Caprolactamase is the first enzyme in the caprolactam degradation pathway of Pseudomonas jessenii. It is composed of two subunits (CapA and CapB) and sequence‐related to other ATP‐dependent enzymes involved in lactam hydrolysis, like 5‐oxoprolinases and hydantoinases. Activity assays with lysates of Escherichia coli cells producing these proteins indicated they are subunits of a caprolactamase (EC 3.5.2.‐x) that catalyzes the first step in the catabolic pathway: the ATP‐dependent hydrolysis of the lactam ring to form 6‐aminocaproic acid (6‐ACA). The crystal structure of caprolactamase shows an (α/β)2 tetramer, with the α subunits (CapA) responsible for ATP‐dependent substrate phosphorylation and the β subunits (CapB) for hydrolytic lactam ring opening.

A 4.0 Å resolution dataset was collected from a single crystal grown in phosphate‐containing Bis‐Tris propane buffer with 20% PEG3350. The structure was solved by molecular replacement and refined to an R/Rfree of 29/37%. The structure shows a (αβ)2 heterotetrameric assembly. The CapB subunits form a dimeric core with an interface area of ca. 1350 Å2 (Pisa server). Each CapB subunit interacts with a CapA subunit on the opposite side of the CapB‐CapB dimer interface, with a buried surface area of ca. 3000 Å2. The structure of CapA is most similar to the ligand‐free state of the homologous acetophenone carboxylase subunit AaApcα (5L9WB 33% sequence identity and RMSD of 2.1 Å). No ATP or ADP was observed in CapAB. The CapB subunit contains 11 long and 5 short α‐helices and 19 β‐strands involved in 5 β‐sheets. Its core structure is similar to that of the α subunit of acetone carboxylase (XaAcα, RMSD 2.3 Å with 580 matched residues) and to the β subunit of acetophenone carboxylase (AaApcβ RMSD of 1.8 Å on 580 residues). The crystal structure of CapAB shows a metal at the expected site in CapB, but the nature of the ion is unknown. However, Zn2+ has a negligible anomalous signal and was therefore tentatively modeled.

>MSKQQYRLGIDAGGTFTDFILADHQGNVQLFKAPSTPHDGTLAIRNGLAQIADALGRTPAEIIADCDLCINGTTVALNALIEKTGVKVGLLCTDGHEDSLEIRLGHKEDGHRYDATYPPAHMLVPRHLRRPIGGRIISDGSEFSPLDEAAIHAAIDYFREQQVQAVAISFVWSVRNPSHEQRAMAMVRAALPDVFVCSGHEVFPQIREYTRTSTTVVNAYLSPVMGRYIERIDALFEELGAQQPTRYFQSNGGLAPGVVMRERAVNAINSGPASAPQAGLCVAQPFGIDNVITVDMGGTSFDITLSKGGRTNFSKDSDFLRYRIGVPMIQVETLGAGGGSIAHLDDFGMLQVGPRSAGANPGPVCYGKGGVEPTVTDANLALGYLADGALLGGSIRLNRQAAIDAIRSKIAEPLGISVERAAVGIITLVNLSMVSGIRRVSIERGYDPRDFALIGAGGAAGMHVMRLAEEIGSKVVLIPKVASGLCAFGQILSDIRYDQLTTLPMRLDDEFVDLEQLNQALQQLRERGMTNLRDDGFGGDNRIECQYSLEIRYLGQIHECSVELSCDRLDRSSLAALRESFHQRHKALFSYSEPNSPVELVNLECSVIARLQRPPMPELATPLKATAAIPAGHRPMLFNAQDDWQDTPVYNGDRIEVGQIIQGPCVIEEATTNILVPPGWRVSLDPSATYELTPGH[2x];>MNTVDPITLAVVRGALETAQREMTLTLEKTSRSSVFNLAHDYSNALFDHLPEMILQGQDIPIHLGSLIPAMKCVAGFFGDEIAEGDVIYHNDPAYMGSHILDCCMYKPVFYKGELVFWTVCKGHLTDIGGPVPAGYNPDAKEIYAEGLRIPPVKLWAQGQRREDVINLLLTNMRARAYQEGDLNAQYGACSVGERHLIELLDRYGVDQVRACITELKDMADRHMRALLRDVPDGFYSGTAILEDSGHGLGELSITAQVEIRGDEAHVLIESPPQVPYFINSYAGNSISGVYLGLMMFAQVPPPYNEGLYRCVSVDLGPSGTLCNAQEPAPHVNCTTTPMETLADAVRLALEQAAPERVTASWGHASGINIAGHDPRNNNDEYVTMVLASVISGAGANKAMDGWPACGPLCCFGALMSGDIELLEYSYPVLIHRYSLMTDSGGAGEFRGGSGTRLELEPLKHAMTVVGFGEGRQLPTAGAAGAKNVLLEPKLGRLIHRHVDGEEDHYIQNTLLTAQPGERVINVNPGGGGYGDPLRRPLATVLADVRNGLVSIDGARLEYGVVIDGNGQLDEAATHAHRAAH[2x]>MSLSPFEHPFLSGLFGDSEIIELFSAKADIDAMIRFETALAQAEAEASIFADDEAEAIVSGLSEFAADMSALRHGVAKDGVVVPELIRQMRAAVAGQAADKVHFGATSQDVIDTSLMLRLKMAAEIIATRLGHLIDTLGDLASRDGHKPLTGYTRMQAAIGITVADRAAGWIAPLERHLLRLETFAQNGFALQFGGAAGTLEKLGDNAGAVRADLAKRLGLADRPQWHNQRDGIAEFANLLSLVTGTLGKFGQDIALMAEIGSEIRLSGGGGSSAMPHKQNPVNAETL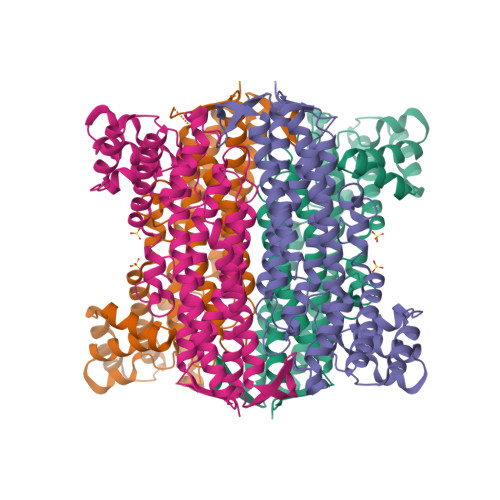VTLARFNAVQISALHQSLVQEQERSGAGWMLEWLTLPQMVTATGTSLLVAERLAAQIDRLGADESHHHHHH[12x]>[7x]MSMYTTAQLLAANEQKFKFDPLFLRLFFRESYPFTTEKVYLSQIPGLVNMALYVSPIVSGEVIRSRGGSTSEFTPGYVK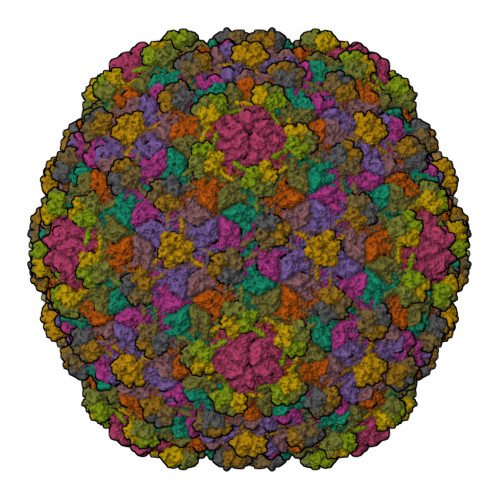PKHEVNPQMTLRRLPDEDPQNLADPAYRRRRIIMQNMRDEELAIAQVEEMQAVSAVLKGKYTMTGEAFDPVEVDMGRSEENNITQSGGTEWSKRDKSTYDPTDDIEAYALNASGVVNIIVFDPKGWALFRSFKAVKEKLDTRRGSNSELETAVKDLGKAVSYKGMYGDVAIVVYSGQYVENGVKKNFLPDNTMVLGNTQARGLRTYGCIQDADAQREGINASARYPKNWVTTGDPAREFTMIQSAPLMLLADPDEFVSVQLA;>[7x]MTSKETFTHYQPQGNSDPAHTATAPGGLSAKAPAMTPLMLDTSSRKLVAWDGTTDGAAVGILAVAADQTSTTLTFYKSGTFRYEDVLWPEAASDETKKRTAFAGTAISIV> MTKTPVAKNGQLQVVGTALLNRDGKPFQLRGISTHGLQWFGQFANKDAFQTLRDDWKANVVRLAMYTDPNANGYIAQPEWLKAKVKEGVEAAKELGMYVIID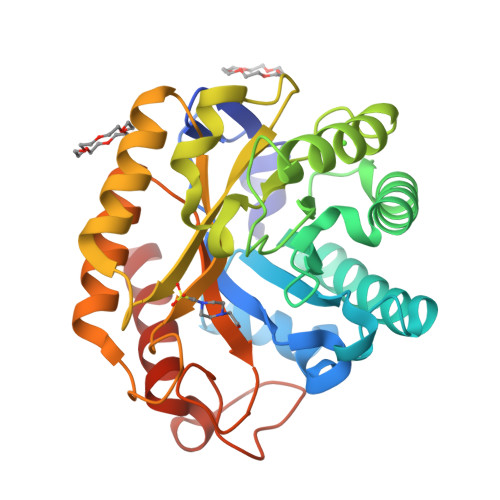WHILNDNDPNLYKEQAKRFFAEMAREYGNTPNVIYEIANEPNGDVTWEEKIRPYADEVIRTIRSIDRDNLIIVGTGTWSQDVDDVASDPLPYKNIMYALHFYAGTHGQFLRDKANYALSKGTPIFVTEWGTSDASGDGGVFLDQSREWLKYLDSKTISWVNWSLCDKNEASAALRPGADPHGGWGDDHLSDSGRFIKAKLIEALEHHHHHH>GQLHLEIAKAPDQAPKIAIVPFNNDNGLYPIVETDLNRSGRFTSSSKNLPANAAINQIQASDWQAAGIPYVVTGQIKQTADGFEVHYQLYDVQKQQYLLNELLNVPASRIRQAGHMVSDAIYQALTGIPGDFSGRIAYVLRNPATPAERYTLQIADTDGEQPKTVLSSRDPILSPAWTPDAKKIAYVSFETKRPAIYLQDLSTGTREVITSFKGLNGAPSFSPDGKSMLFTASMNGNPEIYQMDLSTRQVKRMTNDSGID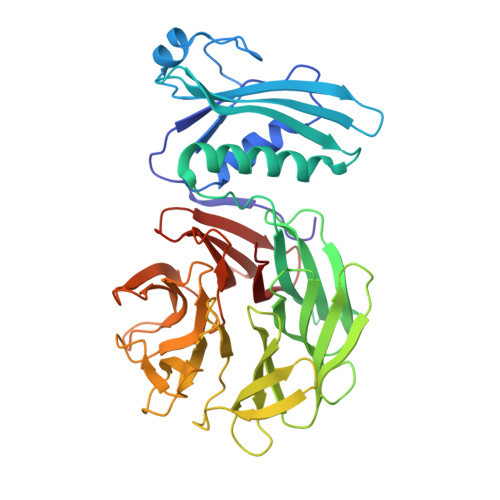TEARYTPDGKAFIFTSDRGGSPQIYRYDFGNGSVKRLTFKGSFNARGTLSADGKKIALVHRPSGSNYKVAIQDINTGIVNILTPTSLDESPSFSPNGQMVVYATREGNRGLLSIMSTDGRFRMNLPSEQGEVREPAWAPK[2x]azepan-2-one | C6 H11 N O | 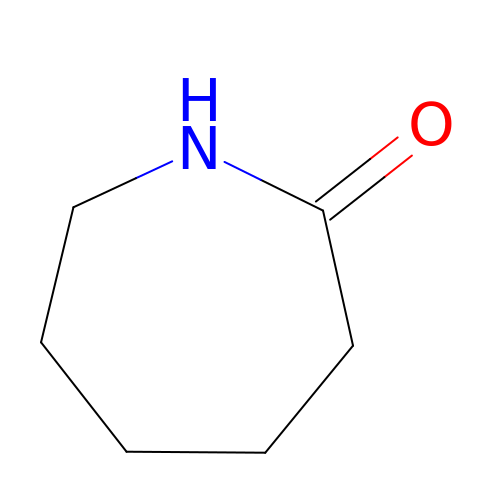JBKVHLHDHHXQEQ-UHFFFAOYSA-N>MSYYHHHHHHLESTSLYKKAGSENLY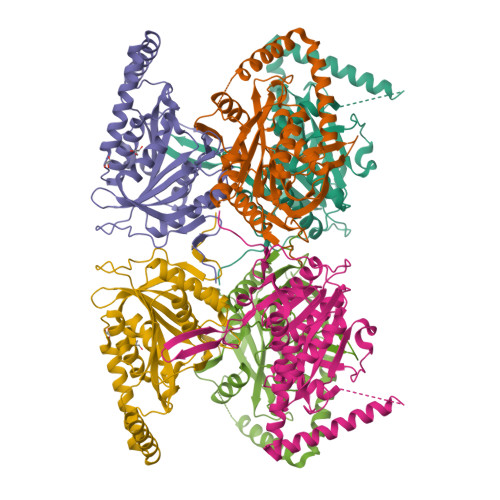FQGARDQGADEAREYEPGQPGMYELEFPAPQLSSSDGRGPVLVHALEGFSDAGHAIRLAAAHLKAALDTELVASFAIDELLDYRSRRPLMTFKTDHFTHSDDPELSLYALRDSIGTPFLLLAGLEPDLKWERFITAVRLLAERLGVRQTIGLGTVPMAVPHTRPITMTAHSNNRELISDFQPSISEIQVPGSASNLLEYRMAQHGHEVVGFTVHVPHYLTQTDYPAAAQALLEQVAKTGSLQLPLAVLAEAAAEVQAKIDEQVQASAEVAQVVAALERQYDAFIDAQENRSLLTRDEDLPSGDELGAEFERFLAQQAEKKSDDDP[3x]> AAGKGKEVLSGVVFQPFEEIKGELSLVPQTPDKSLARQKFVDE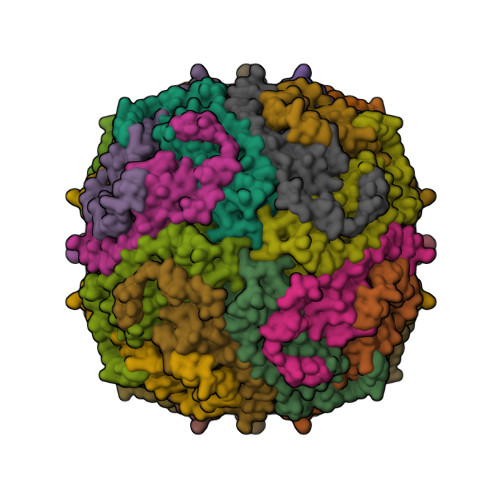CEAAINEQINVEYNASYAYHSLFAYFDRDNVALKGFAKFFKESSDEEREHAEKLMKYQNTRGGRVRLQSIVTPLTEFDHPEKGDALYAMELALALEKLVNEKLHNLHAVATRCNDPQLTDFIESEFLADQVEDIKKISEYVAQLRRVGKGHGVWHFDQKLLEEEA>ILPDSVDWREKGCVTEVKYQGSCGASWAFSAVGALEAQLKLKTGKLVSLSAQNLVDCSTEKYGNKGCNGGFMTTAFQYIIDNKGIDSDASYPYKAMDQKCQYDSKYRAATCSKYTELPYGREDVLKEAVANKGPVSVGVDARHPSFFLYRSGVYYEPSCTQNVNHGVLVVGYGDLNGKEYWLVKNSWGHNFGEEGYIRMARNKGNHCGIASFPSYPEILQGGG[3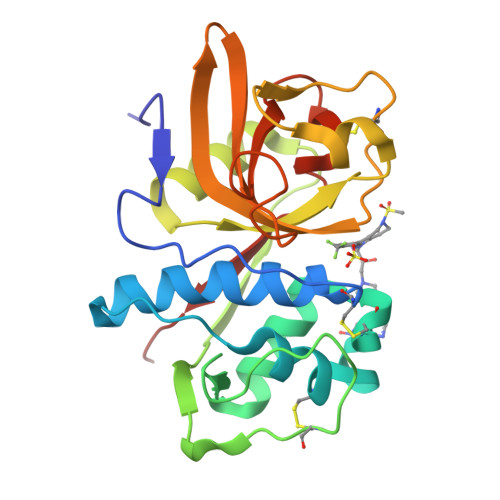x]>MGGEVEEPEPQMVLSPLTSAAIFLVVTIDSGGEDTVRDLLSDVASLERAVGFRAQPDGRLSCVTGIGSEAWDRLFSGARPAGLHPFRELDGPVHRAVATPGDLLFHIRASRLDLCFALATEIMGRLRGAVTPQDEVHGFKYFDERDMLGFVAGTENPTGAAARRAVLVGAEDPAFAGGSYAVVQKYLHDIDAWEGLSVEAQERVIGRRKMTDVELSDDVKPADSHVALTSVTGPDGSDLEILRDNMPFGSVGREEFGTYFIGYARTPEVTETMLERMFLG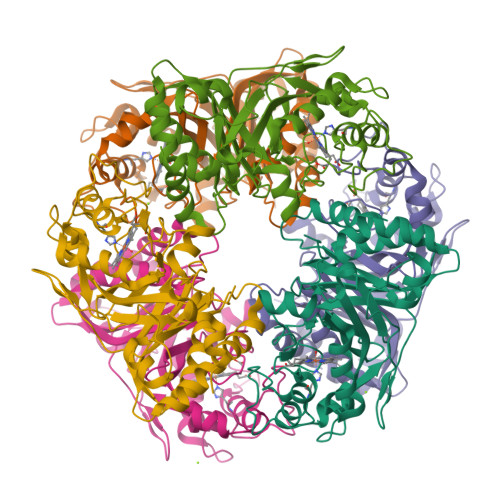TASAPHDRILDFSTAVTGSLFFTPAADFLEDLSARP[6x]> MSNEDYGYDYDYLFKIVLIGDSGVGKSNLLSRFTTDEFNIESKSTIGVEFATRTIEVENKKIKAQIWDTAGQ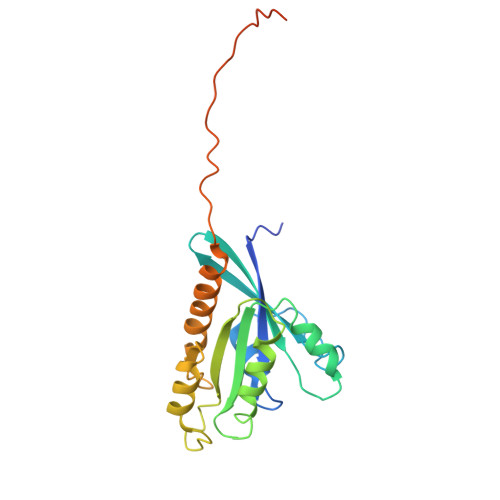ERYRAITSAYYRGAVGALIVYDISKSSSYENCNHWLTELRENADDNVAVGLIGNKSDLAHLRAVPTDEAKNFAMENQMLFTETSALNSDNVDKAFRELIVAIFQMVSKHQVDLSGSGTNNMGSNGAPKGPTISLTPAPKEDKKKKSSNCC> MSKGTTSQDAPFGTLLGYAPGGVAIYSSDYSSLDPQEYEDDAVFRSYIDDEYMGHKWQAVEFARRFLFLNYGVVFTDVGMAWEIFSLRFLREVVNDNILPLQAFPNGSPRAPVAGALLIWDKGGEFKDTGHVAIITQLHGNKVRIAEQ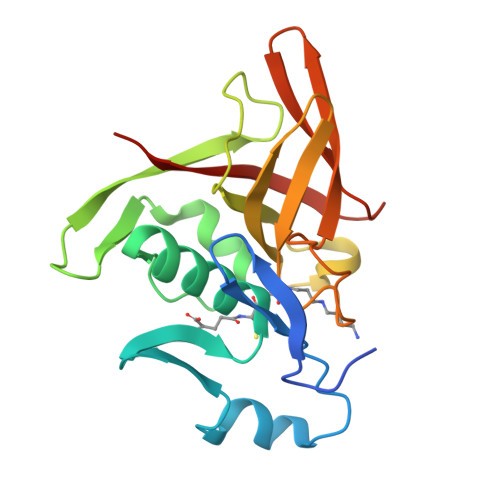NVIHSPLPQGQQWTRELEMVVENGCYTLKDTFDDTTILGWMIQTEDTEY>MSYATKIHARYVYDSRGNPTVEVDFTTDKGLFRSIVPSGASTGVHEALELRDGDKSKWLGKGVLKAVANVNDIIAPALIKAKIDVVDQAKIDEFLLSLDGTPNKSKLGANAILGVSLAAANAAAAAQGIPLYKHIANISNAKKGKFVLPVPFQNVLNGGSHAGGALAFQEFMIAPTGVSTFSEALRIGSEVYHNLKSLTKKKYGQSAGNVGDEGGVAPDIKTPKEALDLIMDAIDKAGYKGKVGIAMDVASSEFYKDGKYDLDFKNPESDPSKWLSGPQLADLYEQLISEYPIVSIEDPFAEDDWDAWVHFFERVGDKIQIVGDDLTVTNPTRIKTAIEKKAANALLLKVNQIGTLTESIQAANDSYAAGWGVMVSHRSGETEDTFIADLSVGLRSGQIKTGAP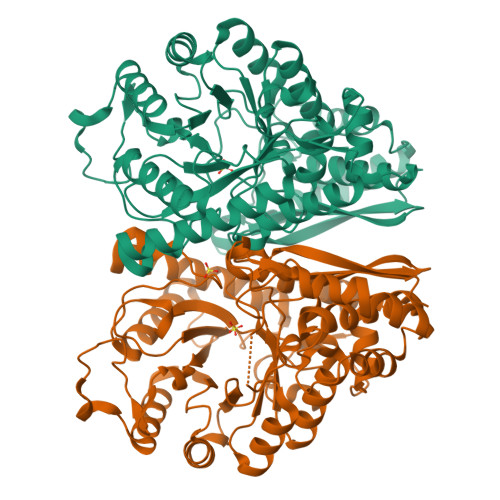ARSERLAKLNQILRIEEELGSEAIYAGKDFQKASQLHHHHHH[4x]> VTRHQVSGWRFVMRRIASGVALHDTRMLVDP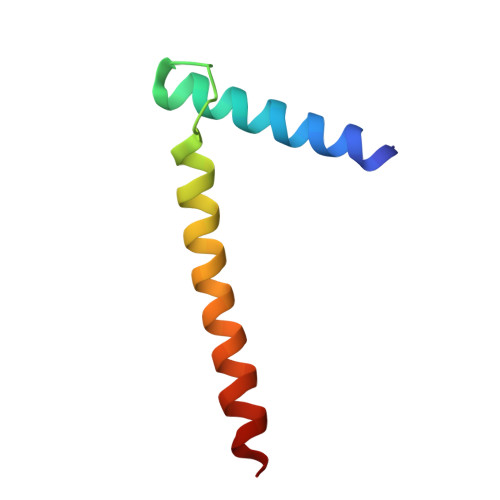LRTQSRAVLTGALILVTGLVGCFIFSLF> GLGDLIEGVVEGVTRNALTPLTPANNLPDTQSSGPAHSKEIPALTAVETGATNPLVPSDTVQTRHVIQKRTRSESTVESFFARGACVAIIEVDNDAPTKRASKLFSVWKITYKDTVQLRRKLEFFTYSRFDMELTFVVTSNYTDANNGHALNQVYQIMFIPPGAPIPGKWNDYTWQTSSNPSVFYTYGAPPARISVPYVGIANAYSHFYDGFAKVPLAGQASTEGDSLYGAASLNDFGSLAVRVVNDHNPTKLTSKIRVYMKPKHVRVWCPRPP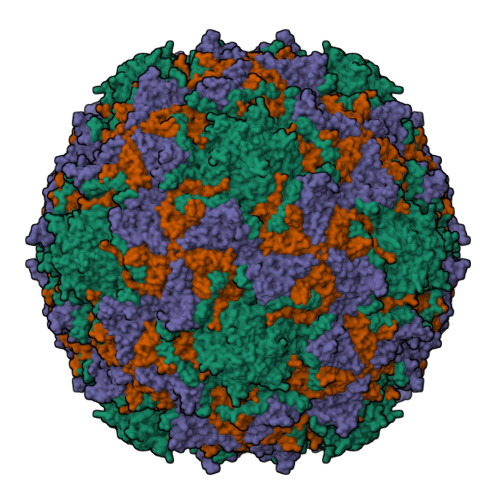RAVPYYGPGVDYKDGLAPLPEKGLTTY;> SPNIEACGYSDRVMQLTLGNSTITTQEAANSVVAYGRWPEYIKDSEANPVDQPTEPDVAACRFYTLDTVTWRKESRGWWWKLPDALKDMGLFGQNMFYHYLGRAGYTVHVQCNASKFHQGALGVFAVPEMCLAGDSTTHMFTKYENANPGEKGGEFKGSFTLDTNATNPARNFCPVDYLFGSGVLAGNAFVYPHQIINLRTNNCATLVLPYVNSLSIDSMTKHNNWGIAILPLAPLDFATESSTEIPITLTIAPMCCEFNGLRNITVPRTQ;> GLPVLNTPGSNQYLTADNYQSPCAIPEFDVTPPIDIPGEVRNMMELAEIDTMIPLNLTNQRKNTMDMYRVELNDAAHSDTPILCFSLSPASDPRLAHTMLGEILNYYTHWAGSLKFTFLFCGSMMATGKLLVSYAPPGAEAPKSRKEAMLGTHVIWDIGLQSSCTMVVPWISNTTYRLTINDSFTEGGYISMFYQTRVVVPLSTPRKMDILGFVSACNDFSVRLLRDTTHISQEAMPQ> MDAAQQGDTTTILMLPWLGYGHLSAFLELAKSLSRRNFHIYFCSTSVNLDAIKPKLPSSFSDSIQFVELHLPSSPEFPPHLHTTNGLPPTLMPALHQAFSMAAQHFESILQTLAPHLLIYDSLQPWAPRVASSLKIPAINFNTTGVFVISQGLHPIHYPHSKFPFSEFVLHNHWKAMYSTADGASTERTRKRGEAFLYCLHASCSVILINSFRELEGKYMDYLSVLLNKKVVPVGPLVYEPNQDGEDEGYSSIKNWLDKKEPSSTVFVSFGSEYFPSKEEMEEIAHGLEASEVNFIWVVRFPQGDNTSGIEDALPKGFLERAGERGMVVKGWAPQAKILKHWSTGGFVSHCGWNSVMESMMFGVPIIGVPMHVDQPFNAG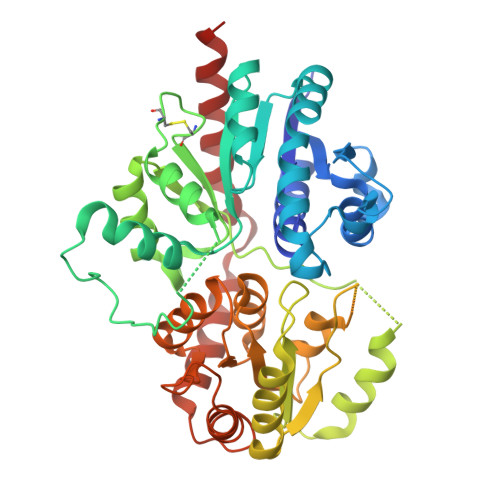LVEEAGVGVEAKRDPDGKIQRDEVAKLIKEVVVEKTREDVRKKAREMSEILRSKGEEKFDEMVAEISLLLKIEHHHHHH>[2x]TETTSFSITKFGPDQQNLIFQGDGYTTKERLTLTKAVRNTVGRALYSSPIHIWDSKTGNVANFVTSFTFVIDAPNSYNVADGFTFFIAPVDTKPQTGGGYLGVFNSKD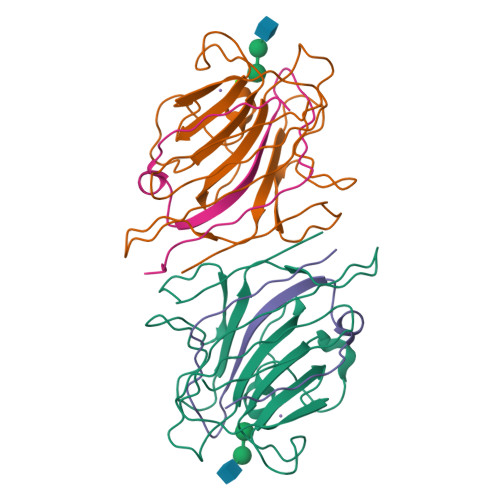YDKTSQTVAVEFDTFYNTAWDPSNGDRHIGIDVNSIKSINTKSWALQNGKEANVVIAFNAATNVLTVSLTYPN;>ETSYTLNEVVPLKEFVPEWVRIGFSATTGAEFAAHEVLSWYFHSELAGTSSS[2x]>GGAAUUGCGGGAAAGGGGUCAACAGCCGUUCAGUA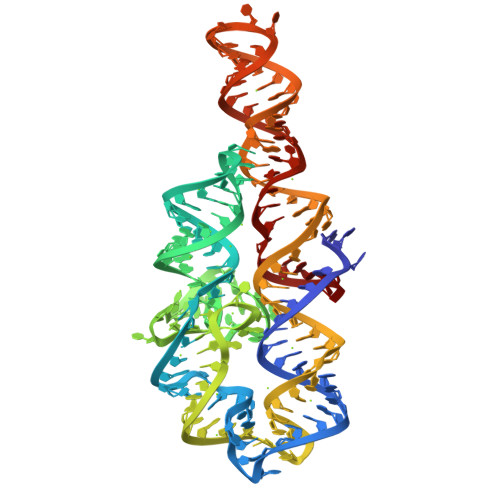CCAAGUCUCAGGGGAAACUUUGAGAUGGCCUUGCAAAGGGUAUGGUAAUAAGCUGACGGACAUGGUCCUAACACGCAGCCAAGUCCUAAGUCAACAGAUCUUCUGUUGAUAUGGAUGCAGUUC[2x]> MAYVEIIEQPKQRGMRFRYKCEGRSAGSIPGERSTDTTKTHPTIKINGYTGP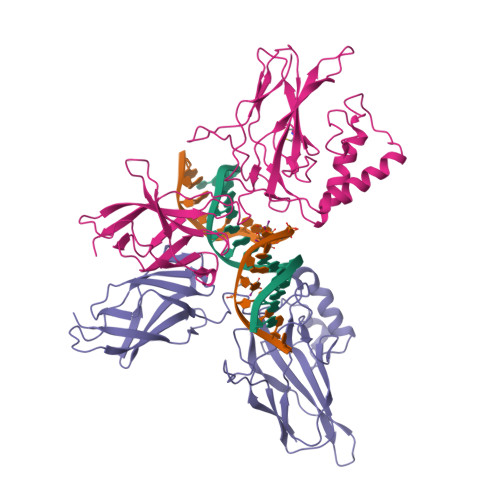GTVRISLVTKDPPHRPHPHELVGKDCRDGYYEADLCPDRSIHSFQNLGIQCVKKRDLEQAISQRIQTNNNPFHVPIEEQRGDYDLNAVRLCFQVTVRDPAGRPLLLTPVLSHPIFDNRAPNTAELKICRVNRNSGSCLGGDEIFLLCDKVQKEDIEVYFTGPGWEARGSFSQADVHRQVAIVFRTPPYADPSLQAPVRVSMQLRRPSDRELSEPMEFQYLPD;> MGPYLQILEQPKQRGFRFRYVCEGPSHGGLPGASSEKNKKSYPQVKICNYVGPAKVIVQLVTNGKNIHLHAHSLVGKHCEDGVCTVTAGPKDMVVGFANLGILHVTKKKVFETLEARMTEACIRGYNPGLLVHSDLAYLQAEGGGDRQLTDREKEIIRQAAVQQTKEMDLSVVRLMFTAFLPDSTGSFTRRLEPVVSDAIYDSKAPNASNLKIVRMDRTAGCVTGGEEIYLLCDKVQKDDIQIRFYEEEENGGVWEGFGDFSPTDVHRQFAIVFKTPKYKDVNITKPASVFVQLRRKSDLETSEPKPFLYYPE>[4x]XSKLE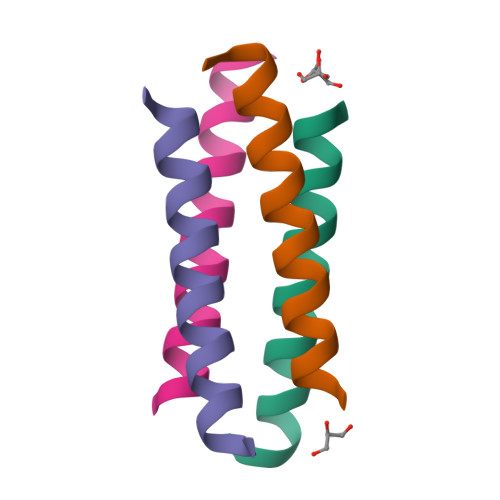ELRRKLQEAEHKARELQEKWGX> KYEYVELAKASLTSAQPQHFYAVVIDATFPYKTNQERYICSLKIVDPTLYLKQQKGAGDASDYATLVLYAKRFEDLPIIHRAGDIIRVHRATLRLYNGQRQFNANVFYSSSWALFSTDKRSVTQEINNQDAVSDTTPFSFSSKHATIEKNEISILQNLRKWANQYFSSYSVISSDMYTALNKAQAQKGDFDVVAKILQVHELDEYTNELKLKDASGQVFYTLSLKLKFPHVRTGEVVRIRSATYDETSTQKKVLILSHYSNIITFIQSSKLAKELRAKIQDDHSVEVASLKKNVSLNAVVLTEVDKKHAALPSTSLQDLFHHADSDKELQAQDTFRTQFYVTKIEPSDVKEWVKGYDRKTKKSSSLKGASGKGDNIFQVQFLVKDASTQLNNNTYRVLLYTQDGLGANFFNVKADNLHKNADARKKLEDSAELLTKFNSYVDAVVERRNGFYLIKDTKLIY;> PQQQSAFKQLYTELFNNEGDFSKVSSNLKKPLKCYVKESYPHFLVTDGYFFVAPYFTKEAVNEFHAKFPNVNIVDLTDKVIVINNWSLELRRVNSAEVFTSYANLEARLIVHSFKPNLQERLNPTRYPVNLFRDDEFKTTIQHFRHTALQAAINKTV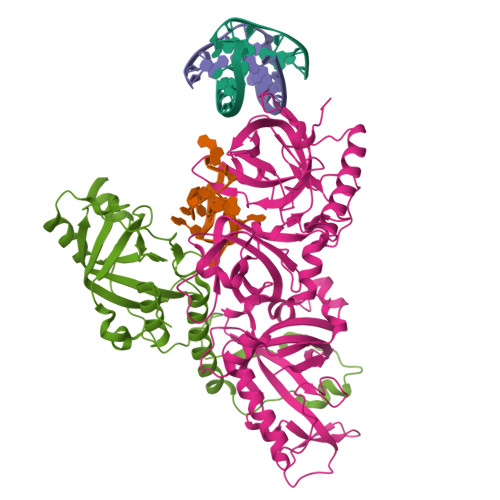KGDNLVDISKVADAAGKKGKVDAGIVKASASKGDEFSDFSFKEGNTATLKIADIFVQEKG>[3x]VAKLVFFAQ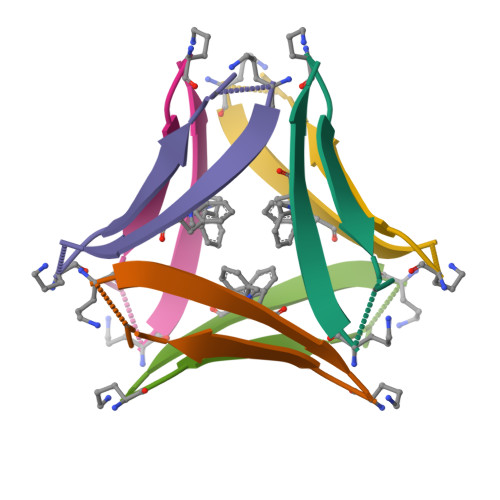AAIIGLM>KEWQENKSWNAHFTEHKSQGVVVLWNENKQQGFTNNLKRANQAFLPASTFKIPNSLIALDLGVVKDEHQVFKWDGQTRDIATWNRDHNLITAMKYSVVPVYQEFARQIGEARMSKMLHAFDYGNEDISGNVDSFWLDGGIRISATEQISFLRKLYHNKLHVSERSQRIVKQAMLTEANGDYIIAAKTGYSTRIEPKIGW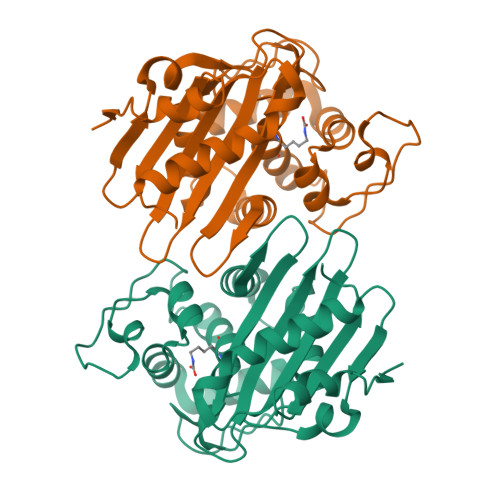WVGWVELDDNVWFFAMNMDMPTSDGLGLRQAITKEVLKQEKIIP[2x]> DMPVERILEAELAVEPDPVTNICQAADKQLFTLVEWAKRIPHFSELPLDDQVILLRAGWN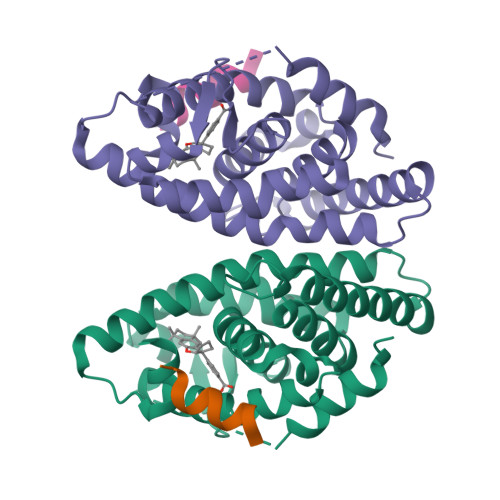ELLIASFSHRSIAVKDGILLATGLHVHRNSAHSAGVGAIFDRVLTELVSKMRDMQMDKTELGCLRAIVLFNPDSKGLSNPAEVEALREKVYASLEAYCKHKYPEQPGRFAKLLLRLPALRSIGLKCLEHLFFFKLIGDTPIDTFLMEMLE;> KHKILHRLLQD> MSTAKAPTLPASIFRAYDIRGVVGDTLTAETAYWIGRAIGSESLARGEPCVAVGRDGRLSGPELVKQLIQGLVDCGCQVSDVGMVPTPVLYYAANVLEGKSGVMLTGAHNPPDYNGFKIVVAGETLANEQIQALRERIEKNDLASGVGSVEQVDILPRYFKQIRDDIAMAKPMKVVVDCGNGVAGVIAPQLIEALGCSVIPLYCEVDGNFPNHHPDPGKPENLKDLIAK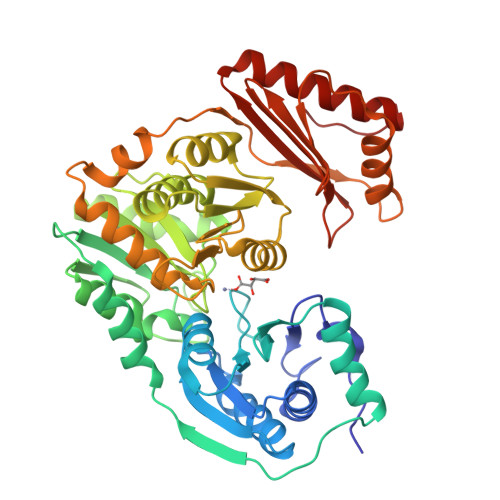VKAENADLGLAFDGDGDRVGVVTNTGTIIYPDRLLMLFAKDVVSRNPGADIIFDVKCTRRLIALISGYGGRPVMWKTGHSLIKKKMKETGALLAGEMSGHVFFKERWFGFDDGIYSAARLLEILSQDQRDSEHVFSAFPSDISTPEINITVTEDSKFAIIEALQRDAQWGEGNITTLDGVRVDYPKGWGLVRASNTTPVLVLRFEADTEEELERIKTVFRNQLKAVDSSLPVPF> ETGCPANCLCSKTDINCKKPDDGNLFPLLEGQDSRNITSIHIENWKNLQTLNAVDMELYTGLQRLTIRNSGLRNIQPRAFAKNPHLRYIDLSGNRLTTLSWQLFQTLRLFDLRLERNPFQCSCDIRWIQLWQEKGEANLQSQQLHCMNLDTAVILLRNMNITQCDLPEISVSHVNLTVREGENAVITCQGSGSPLPDVDWTVADLHSINTHQTNLQWTNVHAIQLTLVNVTSEDNGFLLTCIAEN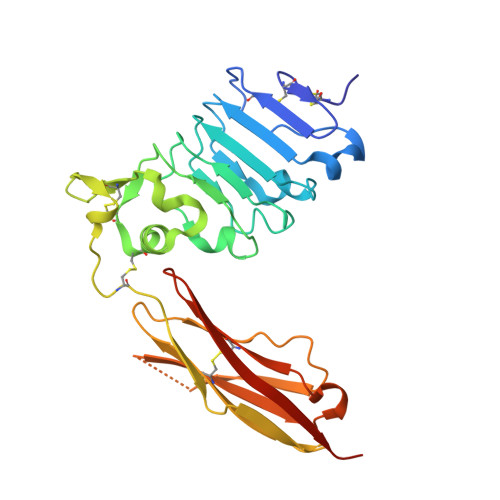VVGMSQASVLLTVYGTKHHHHHH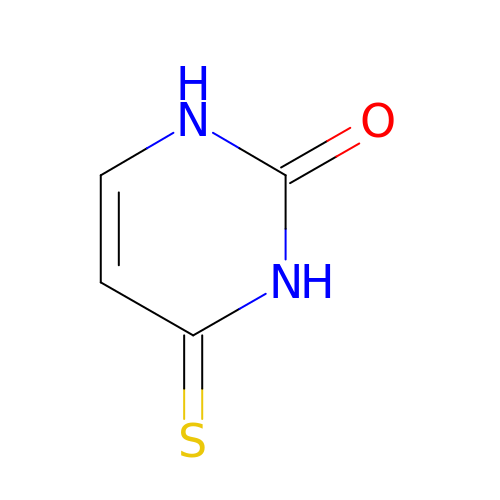4-Thiouracil | C4 H4 N2 O S | OVONXEQGWXGFJD-UHFFFAOYSA-N> MAFSAGAESLLHQAREIQDEELRRFCSRVTKLLQEAPGPATVDALQRLFLIVSATKYPRRLEKMCVDLLQTTLCLPASPEQLQVLCAAILREMSPFNDLALSCDHTPNTRQLSLVASVLLAQGDRKGEIRCVSQRIFKILENRQPEGPSVRPLLPILSKVIGLAPGILMEDQTNLLSKRLVDWLRYASIQQGLPYSGGFFSTPRTRQPGPITEVDGAVASDFFTVLSTGQHFTEDQWVNMQAFSMLRKWLLHSGPEDPCSPDADDKSELEGSTLSVLSAASTASRLLPPRERLREVAFEYCQRLLEQSNRRALRKGDSDLQKACLVEAVSVLDVLCRQDPSFLYRTLSCLKALHRRLGEDPGSERALVPLAQFFLNHGEAAAMDAEAVYGQLLRGLPSERFHSPTLAFEVIHFCTHNLALFDSHFLSLLRLSFPSLFKFLAWNSPPLTAEFVVLLPALVDAGTAVEMLHALLDLPCLTAALDLQLRSTQTPSERLLWDISLRVPSCLEAFQDPQFQGLFRHLLRTKASGSTERLTPLHQVLKPMASCARVTQCAEAVPVLLQAFFSAVTQTADGALINQLALLLLERSDSLYPVPQYEARVHGVLSSQLLVLCKLKPSLVVELSRELLEFVGSVSSIHSRASVFTCVVWAIGEYLSVTWDKRCTAEQINKFFEALEALLFEVTQSRPLADLPCCPPEVVTALMTTLTKLASRSQDLIPRVSLFLSKMRTLAQNPATSSVHSEEGAESIRTRASELLTLLKMPSVAQFVFTPPAGVCQPRYHRDTNVALPLALRTVSRLVEKEAGLLPG;> MGPLSRDAWAQRLGAFRASPSAFMAGPEGEDLGRDLLSDLRSEKLSEQTKVSLLALSMEYPAQLWPDASAAEVAATSLLDTLVLLPPRPSALRRPLLLAATTALAAGGALGPTSGASCRLLPLLLGLAAGSDLGRGFVPASEQRPLQATACECLRELESCKPGLLGGSLGLLRGLLGQEGPVQPLSLLLALALRNTLVLQSRVGAGLGGLLTDKVSPTGGGPWDWTLVEEGDGRLQPQAPSWPAAEEGEGERSLTAREHSPEEARELRAAVIQLLDTSYLLTPVAQAQLLWLLGWALRGLQGQPPALFKPQLVRLLGTAQLTLLHAMLALKAAFGEALFTAQDEALLLRRLTLAAQHPALPPPTHLFYLHCVLSFPENWPLGPEGEEAAPLLLGPQLCRGLLPSLLHDPMALLARLHLLCLLCAEEEEEEKGQLPSPRHYLEELLAGLRQRAALDGGPRALATLCFQASYLVACCLAGQPTVLTPLIHGLAQLYQARPMLAPHFVDLLDQVDSELREPLKVVLRQVVVSRPGRDEALCWHLQMLAKVADGDAQSATLNFLQAAAAHCTNWDLQQGLLRVCRALLRAGVRGGLVDLLQVLARQLEDPDGRDHARLYYILLAHLAAPKLGVALGPSLAAPALASSLVAENQGFVAALMVQEAPALVRLSLGSHRVKGPLPVLKLQPEALEPIYSLELRFRVEGQLYAPLEAVHVPCLCPGRPARPLLLPLQPRCPAPARLDVHALYTTSTGLTCHAHLPPLFVNFADLFLPFPQPPEGAGLGFFEELWDSCLPEGAESRVWCPLGPQGLEGLVSRHLEPFVVVAQPPTSYCVAIHLPPDSKLLLRLEAALADGVPVALRTDDWAVLPLAGDYLRGLAAAV;> MVHAFLIHTLRAPNTEDTGLCRVLYSCVFGAEKSPDDPRPHGAERDRLLRKEQILAVARQVESMCRLQQQASGRPPMDLQPQSSDEQVPLHEAPRGAFRLAAENPFQEPRTVVWLGVLSLGFALVLDAHENLLLAEGTLRLLTRLLLDHLRLLAPSTSLLLRADRIEGILTRFLPHGQLLFLNDQFVQGLEKEFSAAWPR;> MAAEEGVASAASAGGSWGTAAMGRVLPMLLVPVPAEAMGQLGSRAQLRTQPEALGSLTAAGSLQVLSLTPGSRGGGRCCLEGPFWHFLWEDSRNSSTPTEKPKLLALGENYELLIYEFNLKDGRCDATILYSCSREALQKLIDDQDISISLLSLRILSFHNNTSLLFINKCVILHIIFPERDAAIRVLNCFTLPLPAQAVDMIIDTQLCRGILFVLSSLGWIYIFDVVDGTYVAHVDLALHKEDMCNEQQQEPAKISSFTSLKVSQDLDVAVIVSSSNSAVALNLNLYFRQHPGHLLCERILEDLPIQGPKGVDEDDPVNSAYNMKLAKFSFQIDRSWKAQLSSLNETIKNSKLEVSCCAPWFQDILHLESPESGNHSTSVQSWAFIPQDIMHGQYNVLQKDHAKTSDPGRSWKIMHISEQEEPIELKCVSVTGFTALFTWEVERMGYTITLWDLETQGMQCFSLGTKCIPVDSSGDQQLCFVLTENGLSLILFGLTQEEFLNRLMIHGSASTVDTLCHLNGWGRCSIPIHALEAGIENRQLDTVNFFLKSKENLFNPSSKSSVSDQFDHLSSHLYLRNVEELIPALDLLCSAIRESYSEPQSKHFSEQLLNLTLSFLNNQIKELFIHTEELDEHLQKGVNILTSYINELRTFMIKFPWKLTDAIDEYDVHENVPKVKESNIWKKLSFEEVIASAILNNKIPEAQTFFRIDSHSAQKLEELIGIGLNLVFDNLKKNNIKEASELLKNMGFDVKGQLLKICFYTTNKNIRDFLVEILKEKNYFSEKEKRTIDFVHQVEKLYLGHFQENMQIQSFPRYWIKEQDFFKHKSVLDSFLKYDCKDEFNKQDHRIVLNWALWWDQLTQESILLPRISPEEYKSYSPEALWRYLTARHDWLNIILWIGEFQTQHSYASLQQNKWPLLTVDVINQNTSCNNYMRNEILDKLARNGVFLASELEDFECFLLRLSRIGGVIQDTLPVQNYKTKEGWDFHSQFILYCLEHSLQHLLYVYLDCYKLSPENCPFLEKKELHEAHPWFEFLVQCRQVASNLTDPKLIFQASLANAQILIPTNQASVSSMLLEGHTLLALATTMYSPGGVSQVVQNEENENCLKKVDPQLLKMALTPYPKLKTALFPQCTPPSVLPSDITIYHLIQSLSPFDPSRLFGWQSANTLAIGDAWSHLPHFSSPDLVNKYAIVERLNFAYYLHNGRPSFAFGTFLVQELIKSKTPKQLIQQVGNEAYVIGLSSFHIPSIGAACVCFLELLGLDSLKLRVDMKVANIILSYKCRNEDAQYSFIRESVAEKLSKLADGEKTTTEELLVLLEEGTWNSIQQQEIKRLSSESSSQWALVVQFCRLHNMKLSISYLRECAKANDWLQFIIHSQLHNYHPAEVKSLIQYFSPVIQDHLRLAFENLPSVPTSKMDSDQVCNKCPQELQGSKQEMTDLFEILLQCSEEPDSWHWLLVEAVKQQAPILSVLASCLQGASAISCLCVWIITSVEDNVATEAMGHIQDSTEDHTWNLEDLSVIWRTLLTRQKSKTLIRGFQLFFKDSPLLLVMEMYELCMFFRNYKEAEAKLLEFQKSLETLNTAATKVHPVIPAMWLEDQVCFLLKLMLQQCKTQYELGKLLQLFVEREHLFSDGPDVKKLCILCQILKDTSIAINHTIITSYSIENLQHECRSILERLQTDGQFALARRVAELAELPVDNLVIKEITQEMQTLKHIEQWSLKQARIDFWKKCHENFKKNSISSKAASSFFSTQAHVACEHPTGWSSMEERHLLLTLAGHWLAQEDVVPLDKLEELEKQIWLCRITQHTLGRNQEETEPRFSRQISTSGELSFDSLASEFSFSKLAALNTSKYLELNSLPSKETCENRLDWKEQESLNFLIGRLLDDGCVHEASRVCRYFHFYNPDVALVLHCRALASGEASMEDLHPEIHALLQSAELLEEEAPDIPLRRVHSTSSLDSQKFVTVPSSNEVVTNLEVLTSKCLHGKNYCRQVLCLYDLAKELGCSYTDVAAQDGEAMLRKILASQQPDRCKRAQAFISTQGLKPDTVAELVAEEVTRELLTSSQGTGHKQMFNPTEESQTFLQLTTLCQDRTLVGMKLLDKISSVPHGELSCTTELLILAHHCFTLTCHMEGIIRVLQAAHMLTDNHLAPSEEYGLVVRLLTGIGRYNEMTYIFDLLHKKHYFEVLMRKKLDPSGTLKTALLDYIKRCRPGD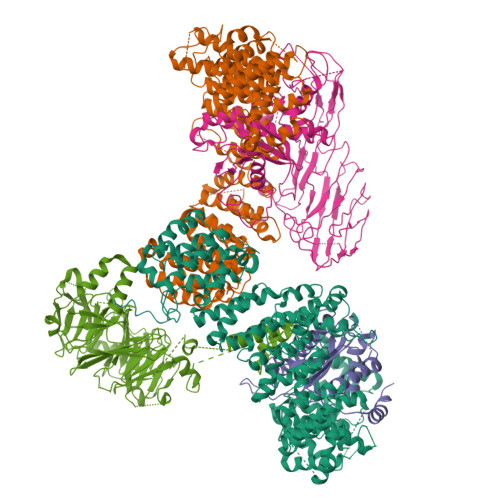SEKHNMIALCFSMCREIGENHEAAARIQLKLIESQPWEDSLKDGHQLKQLLLKALTLMLDAAESYAKDSCVRQAQHCQRLTKLITLQIHFLNTGQNTMLINLGRHKLMDCILALPRFYQASIVAEAYDFVPDWAEILYQQVILKGDFNYLEEFKQQRLLKSSIFEEISKKYKQHQPTDMVMENLKKLLTYCEDVYLYYKLAYEHKFYEIVNVLLKDPQTGCCLKDMLAG;> MALRAVWLIRHEPGTPLGGTVRFSRRYPTVEKRAKAFNGMTYVPVPEDGPFLRALLFQLRLLDDDKDFMERRDGCSRINKTSIYGLSVGGEELWPVIAFLRDSMIYASVPLVEQALSPRPPLISISGVSQGLELLLGIQDFLYSSQKNDTDLHTKLSQLPDLLLQACPLGTLLDANLQNSLNSINSVSVTQPQKQPAWKVGAYKGKAQISISITETVKCMQYGKQDIADTWQVAGTVACKCDLEGVMPAVTISLSLPTNGSPLQDIIVHPCVTSLDSAILTSSSIDTMDDSAFSGPYKFPFTPPLESFNLCHYTSQVPVPPILGSYHMKEEGVQLKVTVNFKLHESVRNNFEVCEAHIPFYNRGPITHLEYKASFGQLEVFREKSLLVWIIGQKFPKSMEISLSGTLTFGVKGHNKQPFDHICIGNTAYIKLNFRIADYTLTGCYADQHSVQVFASGKPKISAYRKLISSDYYIWNSKAPAPVTYASLLP>[6x]AQPGRKLGYAILGLGYYATRIIMPRFAECEHSRLAALVSGTPEKLKTYGEQYGIPETHRYSYETFDRIIDNPDVDIVYVITPNSLHRPFTERAARAGKHVMCEKPMANTVADCEAMIAACKKAGRKLMIGYRSRFQAHNIEAIKLVRDGALGPVRTVVTDHGFTIGDPKQWRLNRALAGGGSLMDIGIYSLNAARYLTGEEP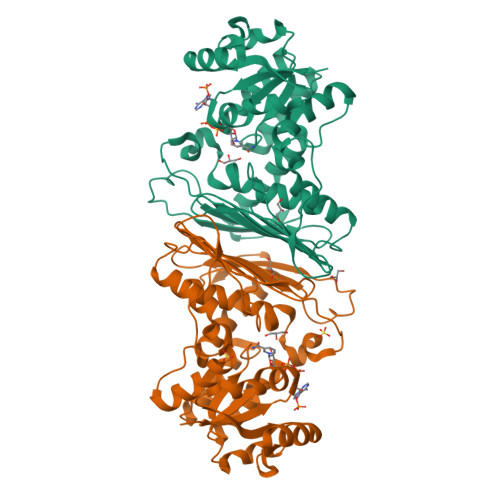VAVNAVESTDRSDPRFGEVEDIINFQLLFPSGATANCVSAYSVNCNRYRVSGPKGWVEIDPATSYQGQAMRAQLGGPPAPREPAPQPKNQFSAQLDHLSECILTGREPIVGGDDGLKDLRVIEAIYRAAREGRTVKL> QALLFPLCLVLYTFSTYIGNMMIQPGMLAVVEQYQAGIDWVPTSMTAYLAGGMFLQWLLGPLSDRIGRRPVMLAGVVWFIVTCLAILLAQNIEQFTLLRFLQGISLCFIGAVGYAAIQESFEEAVCIKITALMANVELIAPLLGPLVGAAWIHVLPWEGMFVLFAALAAISFFGLQRAMPETATRIGEKLSLKELGRDYKLVLKNGRFVAGALALGFVSLPLLAWIAQSPIIIITGEQLSSYEYGLLQVPIFGALIAGNLLLARLTSRRTVRSLIIMGGWPIMIGLLVAAAATVISSHAYLWMTAGLSIYAFGIGLANAGLVRLTLFASDMSKGTVSAAMGMLQMLIFTVGIEISKHAWLNGGNGLFNLFNLVNGILWLSLMVIFLK

By contrast, MdfA from Escherichia coli, a polyspecific MFS multidrug transporter in the ubiquitous drug/H+ antiporter-1 (DHA1) subfamily, can export physicochemically disparate compounds that lack a common chemical structure. Moreover, the coupling between drug binding and deprotonation in MdfA is surprisingly flexible, as a functional MdfA variant can be produced by simply rearranging the substrate- and H+-binding protein residues. Toward this goal, we carried out structural and functional studies of a triple mutant of MdfA, E26T/D34M/A150E, in which the substrate binding and protonation sites are rearranged and yet the multidrug transport function is retained. Our results revealed how this redesigned bacterial multidrug transporter interacts with different substrates and suggested how the antiport function of MdfA tolerates the rearrangement of both drug-binding and protonation sites.

The best diffracting crystals of E26T/D34M/A150E were obtained in the presence of chloramphenicol (Cm), an electroneutral substrate, at pH 8.0. The resulting structure of E26T/D34M/A150E has been refined to 2.0 Å resolution and revealed a transporter structure that is similar to that of Cm-bound MdfA variant Q131R22, with an rms deviation of 1.0 Å for 387 common Cα atoms. Q131R is a fortuitous single mutant that was identified during the crystallographic pursuit of ligand-bound MdfA, which likely represents the wild type transporter when protein-ligand interactions are analyzed. This structural similarity suggested that our E26T/D34M/A150E structure portrays the transporter in its inward-facing conformation and the triple mutation E26T/D34M/A150E did not perturb the protein structure to any significant degree. Located approximately halfway across the membrane bilayer, the bound Cm engages in a number of close-range interactions with the transporter. Specifically, the O4, O5 and CL1 atoms in Cm form direct H-bonds with the side-chains of A150E (OE1), Q357 (NE2) and S232 (OG), respectively. Moreover, the bound Cm makes van der Waals interactions with the side chains of L236 and F361. In addition, the nitrobenzene moiety of Cm appears to interact favorably with the side-chain phenol of Y30, since the electronegative nitryl group of Cm is 3.3 Å from the electropositive edge of the aromatic ring in Y30. Thus, given the pH (8.0) of the crystal solutions, our Cm-bound structure of E26T/D34M/A150E likely portrays a substrate-bound, deprotonated transporter. By contrast, the bound Cm is 3.0 Å from A150 in E26T/D34M/A150E at pH 8.0.>GPPGPPGP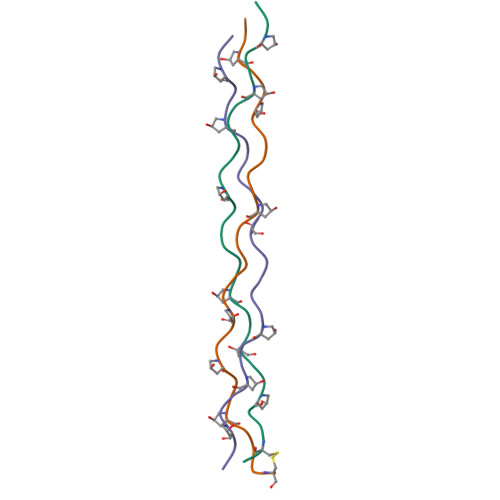RGQPGVMGFPGPPGPPGPCCGGV[3x]>GSGTDNNHYENNESNENSSENSKVDEARAGAFERFTNRKKRFRENAQKNGESSHHEAPSHHKKEHRPNKKPNNHHKQKHAKTRNYAKEELDSNKVEGVTEILHVNERGTLGFHKELKKGVETNNKIQVEHLNPHYKMNLNSKASVKITPLGGLGEIGGNMMVIETPKSAIVIDAGMSFPKEGLFGVDILIPDFSYLHQIKDKIAGIIITHAHEDHIGATPYLFKELQFPLYGTPLSLGLIGSKFDEHGLKKYRSYFKIVEKRCPISVGEFIIEWIHITHSIIDSSALAIQTKAGTIIHTGDFKIDHTPVDNLPTDLYRLAHYGEKGVMLLLSDSTNSHKSGTTPSESTIAPAFDTLFKEAQGRVIMSTFSSNIHRVYQAIQYGIKYNRKIAVIGRSMEKNLDIARELGYIHLPYQSFIEANEVAKYPDNEVLIVTTGSQGETMSALYRMATDEHRHISIKPNDLVIISAKAIPGNEASVSAVLNFLIKKEAKVAYQEFDNIHVSGHAAQEEQKLMLRLIKPKFFLPVHGEYNHVARHKQTAISCGVPEKNIYLMEDGDQVEVGPAFIKKVGTIKSGKSYVDNQSNLSIDTSIVQQREEVASAGVFAATIFVNKNKQALLESSQFSSLGLVGFKDEKPLIKEIQGGLEMLLKSSNAEILNNPKKLEDHTRNFIRKALFKKFRK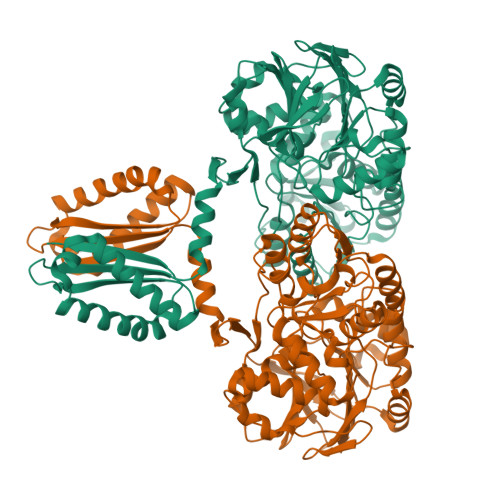YPAIICHAHSFGSSPHHHHHHHH[4x]> MRGSHHHHHHGSMAVPPTYADLGKSARDVFTKGYGFGLIKLDLKTKSENGLEFTSSGSANTETTKV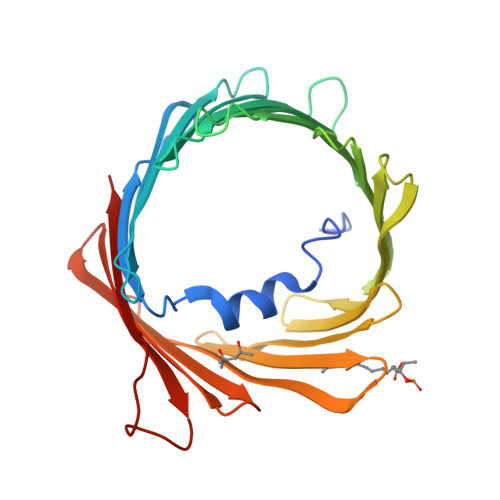NGSLETKYRWTEYGLTFTEKWNTDNTLGTEITVEDQLARGLKLTFDSSFSPNTGKKNAKIKTGYKREHINLGCDVDFDIAGPSIRGALVLGYEGWLAGYQMNFETSKSRVTQSNFAVGYKTDEFQLHTNVNDGTEFGGSIYQKVNKKLETAVNLAWTAGNSNTRFGIAAKYQVDPDACFSAKVNNSSLIGLGYTQTLKPGIKLTLSALLDGKNVNAGGHKLGLGLEFQA> GRKEKVVLKIASIAPARSIWETELKKLSAEWSEITGGLVSMKFYDMSSLGGEREGIRKLKSSRPGQAAPLDGAVFSCLGLSELAPDSGIYTLSVPFLIQNEKDLERVLHELREDLDRPFRAAGFRVITWTNAGWLSF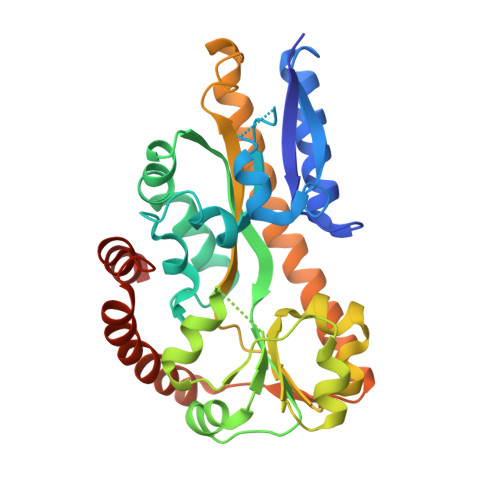YTRAPYASLGQLKKQTIALSSLDSSVLGTCFRICGFDIKDAPNVRLAPLLKAGSIDGFLSVHLFTWATGFYRYISYALDTKICPAVIGMLISDGSWARIPSRYHDAMLQAATRVRQRLANNLETLDRECSNNIQKAGVSIVHLTPQEIQEWRTEFAADVKRIQARLPGMLNMTLYEKIKHLLYSAQR>[2x]LDLFVSPLGRVEGDLDVRVTINDGVVTSAWTEAAMFRGFEIILRGKDPQAGLIVCPRICGICGGSHLYKSAYALDTAWRTHMPPNATLIRNICQACETLQSIPRYFYALFAIDLTNKNYAKSKLYDEAVRRFAPYVGTSYQPGVVLSAKPVEVYAIFGGQWPHSSFMVPGGVMSAPTLSDVTRAIAILEHWNDNWLEKQWLGCSVDRWLENKTWNDVLAWVDENESQYNSDCGFFIRYCLDVGLDKYGQGVGNYLATGTYFEPSLYENPTIEGRNAALIGRSGVFADGRYFEFDQANVTEDVTHSFYEGNRPLHPFEGETIPVN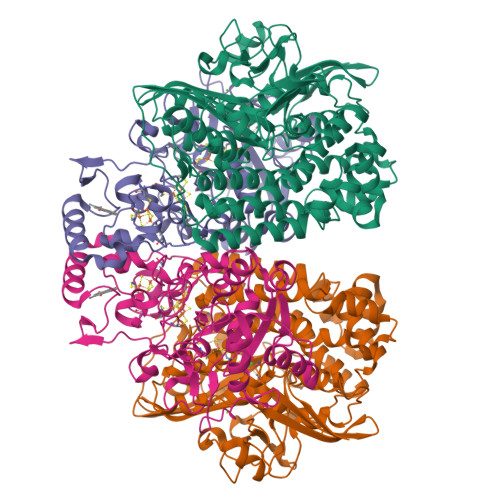PEDGRRQGKYSWAKSPRYAVPGLGNVPLETGPLARRMAASAPDAETHQDDDPLFADIYNAIGPSVMVRQLARMHEGPKYYKWVRQWLDDLELKESFYTKPVEYAEGKGFGSTEAARGALSDWIVIEDSKIKNYQVVTPTAWNIGPRDASEVLGPIEQALVGSPIVDAEDPVELGHVARSFDSCLVCTVH;>ASVLWFQGGACSGNTMSFLNADEPNVVDLIVDFGLDLLWHPSLGLELGNNAQKVFWDCAKGERPLDIFVFEGTVIEAPNGTGQMDMFAGRPMKDWVTDLAGAAQIVVAIGDCACFGGIPAMEPNPSGSTGLQFHKREKGGFLGPDFRSKMGLPVINVPGCPAHPDWITQILVALATGRAGDITLDDLHRPETFFKTFTQTGCTRVQFFEYKQSTLSFGEGTRTGCLFYEFGCRGPMTHSPCNRILWNRQSSKTRAGMPCLGCTEPEFPHFDLAPGTVFKTQKVSGMIPKEVPEGTDHLTYMGLAAAARIAAPQWSKEDMFVV[2x]>[2x]ESCHPRLSLHRPALEDLLLGSEANLTCTLTGLRDASGVTFTWTPSSGKSAVQGPPERDLCGCYSVSSVLPGCA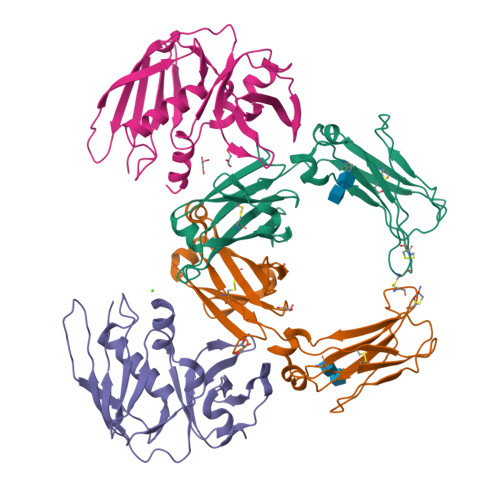EPWNHGKTFTCTAAYPESKTPLTATLSKSGNTFRPEVHLLPPPSEELALNELVTLTCLARGFSPKDVLVRWLQGSQELPREKYLTWASRQEPSQGTTTFAVTSILRVAAEDWKKGDTFSCMVGHEALPLAFTQKTIDRLAGKP;>KEKQERVQHLYDIKDLHRYYSSESFEFSNISGKVENYNGSNVVRFNQEKQNHQLFLLGEDKAKYKQGLQGQDVFVVKELIDPNGRLSTVGGVTKKNNQSSETNIHLLVNKLDGGNLDATNDSFLINKEEVSLKELDFKIRKQLVEKYGLYQGTSKYGKITIILNGGKKQEIDLGDKLQFERMGDVLNSKDINKIEVTLKQI[2x]>[2x]MIKLCIAGKNNIAVNSLEYILKNHFKPDQVAVIPNKNDFGVDSWQKSLLHYAFNNHIKVITLEEAYELKQIIFFSLEFDRIVKVEKFKSDKLFNMHFSALPKYKGVFTSITPILNNEVESGVTLHCIDNGIDTGNIIDQYIFPININDTARDLYFNYLSYGEYLFKKNIQRIINNTYENFKQNNISSSYFSRQDININHKINFKKTSFEIHNQIRAFIFKEYQLPSINKTKIIK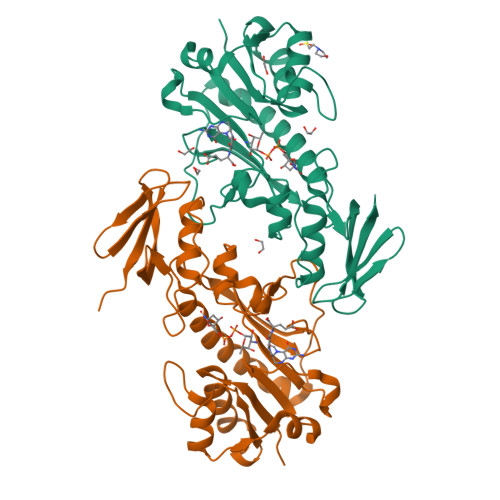STLTNEFIGYNMFEEFEEYFMISGIDGFKIIAQKYNAELEHHHHHH We have characterized a glycoside hydrolase 5 (GH5) domain of a bi-catalytic GH5-GH6 multi-domain enzyme from the unusual gill endosymbiont Teredinibacter waterburyi of the wood-digesting shipworm Psiloteredo megotara. The enzyme is part of a large multi-domain cellulase comprised of a N-terminal GH5 domain, followed by three CBM10 domains separated by serine-rich linker region and a C-terminal GH6 domain. The results showed that TwCel5 is an endo-β-1,4-glucanase with a catalytic properties that renders it a potentially attractive industrial biocatalyst for cellulose bioconversion. Furthermore, products generated from enzymatic hydrolytic of PASC by HPAEC-PAD analysis revealed cellobiose as predominant product with lesser amount of glucose, and cellotriose, as is commonly observed for cellulases. In summary, the observed activities, product distribution, and cleavage patterns strongly indicate that TwCel5 is a β-(1,4)-endo-glucanase with a mode of action resembling that of other known GH5 enzymes.

To gain structural insights for TwCel5CAT, bond cleavage pattern and mode of action, we solved and determined the tertiary structure of the catalytic module. TwCel5CAT was crystallized in an apo form and a dataset diffracting to 1.0 Å resolution was collected. The crystal structure of the GH5 catalytic domain was solved to 1.0 Å resolution and revealed a substrate binding cleft extension containing a putative + 3 subsite, which is uncommon in this enzyme family. Consistent with the defining family member, TwCel5CAT exhibits a classical (β/α)8-barrel fold (also known as TIM-barrel) with two conserved glutamates; Glu157 & Glu245 in the catalytic center that are positioned to promote the expected displacement mechanism characteristic of family 5 cellulases. Thus, from homology to other GH family 5 cellulases, the proton donor is expected to be Glu157, and the nucleophile is Glu228. Furthermore, substrate binding cleft of TwCel5CAT is similar to other clade 2 GH5 enzymes, showing conserved aromatic and polar amino acids involved in substrate binding. In contrast to most other GH5s subfamily 2, TwCel5CAT has a tryptophan (Trp226) in the outer region of the reducing end subsites. Of the 15 unique structures from GH5s subfamily 2, only three have a Trp in this position, namely the thermostable GsCelA from Geobacillus sp. 70PC53, the halotolerant Cel5R cloned from a soil metagenome and Cel5B from C. hutchinsonii, respectively. Of note, a comparison of the Alphafold2 model of TwCel5CAT with the X-ray crystallographic structure showed RMSD for Cα-carbons of only 0.35 Å. Furthermore, the side chains of the amino acids in the conserved active site and substrate binding cleft were modelled close to flawlessly.

> MISNKVKSLFATAAAAVFATSVAVMDVPAVSVSGNQVLFGGQAKSLAGNSFFWSNTGWGQERFYTAETVRWLKSDFKASIVRASMGVDDEGGYLEDASNKTRIETVVDAAIAEDLYVIIDWHSHHAEDYRAESIAFFEEMARKYGNNNHVIYEIYNEPLQISWSNTIKPYAEAVIGAIRAIDPDNLIIVGTPSWSQDVDAASNDPITSYSNIAYTLHFYAGTHQQWLRDKATTAMNNGIALFATEWGTVDADGDGAVNRSETNAWMDFFKQNNISHANWVISDKAEGSSLVNPNAPVSGWSSSDLTESGNFVRDIVRNWGA4-oxidanylbenzohydrazide | C7 H8 N2 O2 | 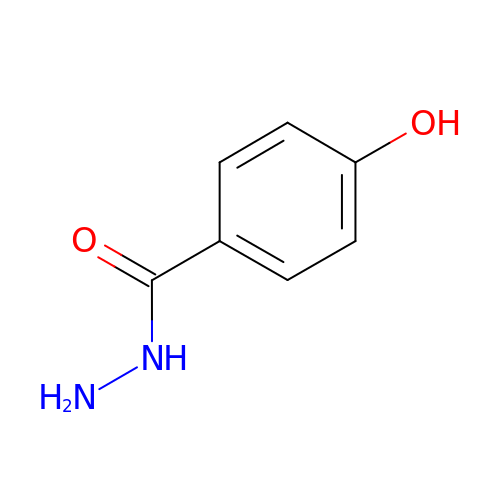ZMZGIVVRBMFZSG-UHFFFAOYSA-N4'-fluoro-6-(trifluoromethyl)[1,1'-biphenyl]-2-yl 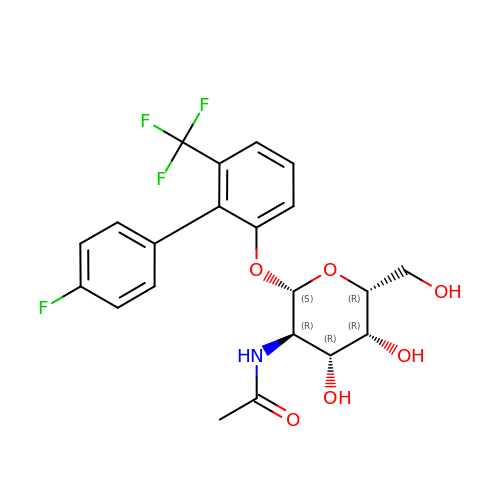2-acetamido-2-deoxy-beta-D-galactopyranoside | C21 H21 F4 N O6 | HRLDWJXNEKTIOQ-XIKSMUEASA-N>MKKGVLIAFEGIDGSGKSSQATLLKDWIELKRDVYLTEWNSSDWIHDIIKEAKKKDLLTPLTFSLIHATDFSDRYERYILPMLKSGFIVISDRYIYTAYARDSVRGVDIDWVKKLYSFAIKPDITFYIRVSPDIALERIKKSKRKIKPQEAGADIFPGLSPEEGFLKYQGLITEVYDKLVKDENFIVIDGTK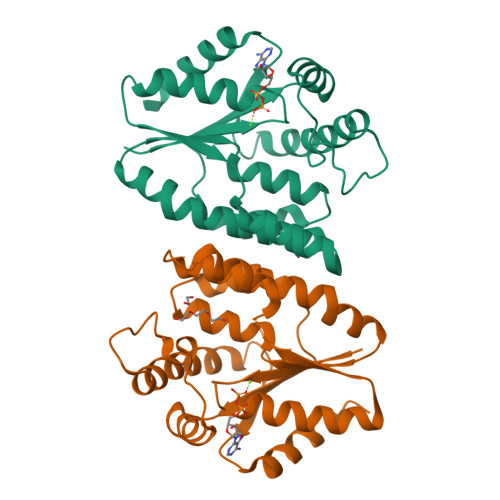TPKEIQIQIRKFVGELIDNSF[2x]> MIDVIMTGELLKTVTRAIVALVSEARIHFLEKGLHSRAVDPANVAMVIVDIPKDSFEVYNIDEEKTIGVDMDRIFDISKSISTKDLVELIVEDESTLKVKFGSVEYKVALIDPSAIRKEPRIPELELPAKIVMDAGEFKKAIAAADKISDQVIFRSDKEGFRIEAKGDVDSIVFHMTETELIEFNGGEARSMFSVDYLKEFCKVAGSGDLLTIHLGTNYPVRLVFELVGGRAKVEYILAPRI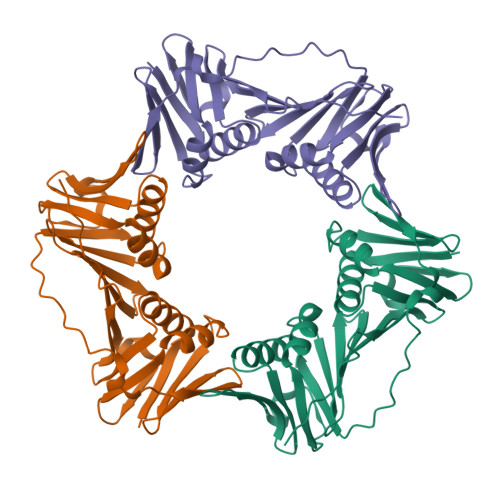ESE> IKVGINGFGRIGRIVFRAAQKRSDIEIVAINDLLDADYMAYMLKYDSTHGRFDGTVEVKDGHLIVNGKKIRVTAERGPANLKWDEVGVDVVAEATGLFLTDETARKHITAGAKKVVMTGPSKDNTPMFVKGANFDKYAGQDIVSNASCTTNCLAPLAKVINDNFGIIEGLMTTVHATTATQKTVDGPSHKDWRGGRGASQNIIPSSTGAAKAVGKVLPELNGKLTGMAFRVPTPNVSV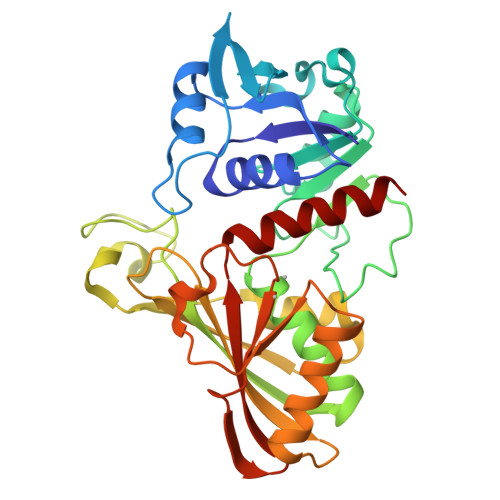VDLTVRLEKAATYEQIKAAVKAAAEGEMKGVLGYTEDDVVSTDFNGEVCTSVFDAKAGIALNDNFVKLVSWYDNETGYSNKVLDLIAHISK> MKQALRVAFGFLILWASVLHAEVRIVIDSGVDSGRPIGVVPFQWAGPGAAPEDIGGIVAADLRNSGKFNPLDRARLPQQPGSAQEVQPAAWSALGIDAVVVGQVTPNPDGSYNVAYQLVDTGGAPGTVLAQNSYKVNKQWLRYAGHTASDEVFEKLTGIKGAFRTRIAYVVQTNGGQFPYELRVSDYDGYNQFVVHRSPQPLMSPAWSPDGSKLAYVTFESGRSA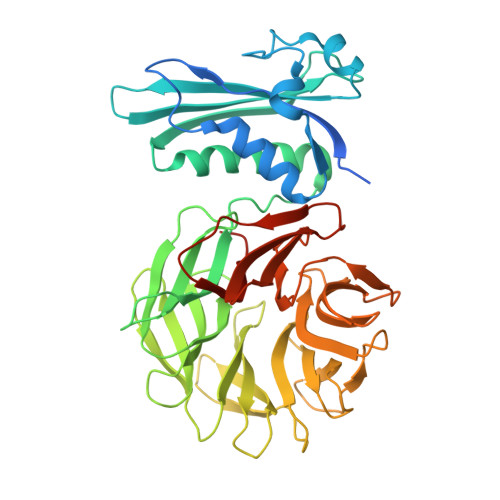LVIQTLANGAVRQVASFPRHNGAPAFSPDGSKLAFALSKTGSLNLYVMDLASGQIRQVTDGRSNNTEPTWFPDSQNLAFTSDQAGRPQVYKVNINGGAPQRITWEGSQNQDADVSSDGKFMVMVSSNGGQQHIAKQDLATGGVQVLSSTFLDETPSLAPNGTMVIYSSSQGMGSVLNLVSTDGRFKARLPATDGQVKFPAWSPYLLEHHHHHH>MQRVTITLDDDLLETLDSLSQRRGYNNRSEAIRDILRSALAQEATQQHGTQGFAVLSYVYEHEKRDLASRIVSTQHHHHDLSVATLHVHI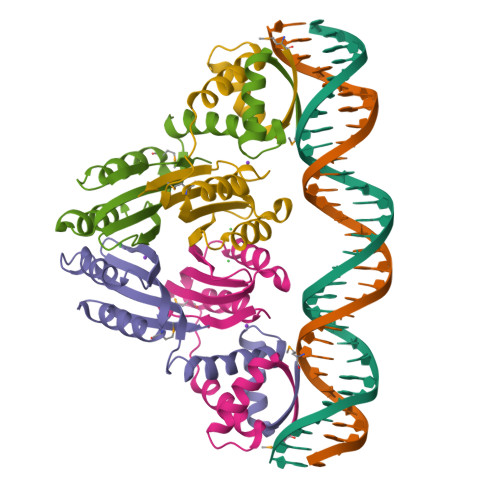NHDDCLEIAVLKGDMGDVQHFADDVIAQRGVRHGHLQCLPKED[8x]> DQYEYKYPAIKDLKKPCITLGKAPDLNKAYKSVLSGMNAAKLDPDDVCSYLAAAMQFFEGTCPEDWTSYGILIARKGDRITPNSLVEIKRTDVEGNWALTGGMELTRDPTVSEHASLVGLLLSLYRLSKISGQNTGNYKTNI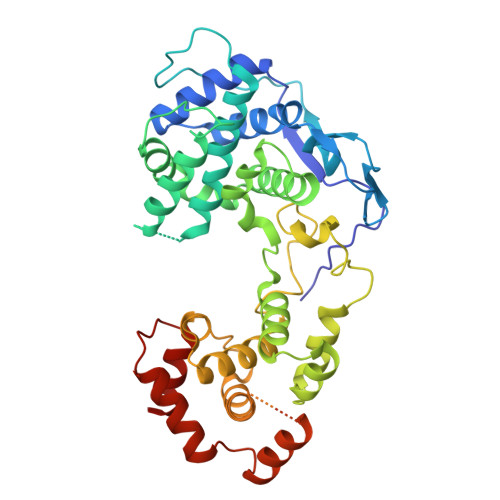ADRIEQIFETAPFVKIVEHHTLMTTHKMCANWSTIPNFRFLAGTYDMFFSRIEHLYSAIRVGTVVTAYEDCSGLVSFTGFIKQINLTAREAILYFFHKNFEEEIRRMFEPGQETAVPHSYFIHFRSLGLSGKSPYSSNAVGHVFNLIHFVGCYMGQVRSLNATVIAACAPHEMSVLGGYLGEEFFGKGTFERRFFRDEKELQEYEAAELTKSDVALADDGTVNSDDEDYFSGETRSPEAVYTRIMMNGGRLKRSHIRRYVSVSSNHQARPNSFAEFLNKTYSNDS> MESLTLQPIARVDGTINLPGSKSVSNRALLLAALAHGKTVLTNLLDSDDVRHMLNALTALGVSYTLSADRTRCEIIGNGGPLHAEGALELFLGNAGIAMRSLAAALCLGSNDIVLTGEPRMKERPIGHLVDALRLGGAKITYLEQENYPPLRLQGGFTGGNVDVDGSVSSQFLTALLMTAPLAPEDTVIRIKGDLVSKPYIDITLNLMKTFGVEIENQHYQQFVVKGGQSYQSPGTYLVEGDASSASYFLAAAAIKGGTVKVTGIGRNSMQGDIRFADVLEKMGATICWGDDYISCTRGELNAIDMDMNHIPDAAMTIATAALFAKGTTTLRNIYNWRVKETDRLFAMATELRKVGAEVEEGHDYIRITPPEKLNFA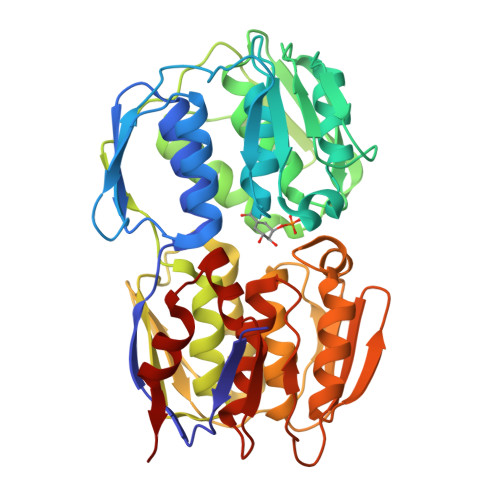EIATYNDHRMAMCFSLVALSDTPVTILDPKCTAKTFPDYFEQLARISQAA>MSTRSARIVVVSSRAAAGVYTDDCGPIIAGWLEQHGFSSVQPQVVADGNPVGEALHDAVNAGVDVIITSGGTGISPTDTTPEHTVAVLDYVIPGLADAIRRSGLPKVPTSVLSRGVCGVAGRTLIINLPGSPGGVRDGLGVLADVLDHALEQIAG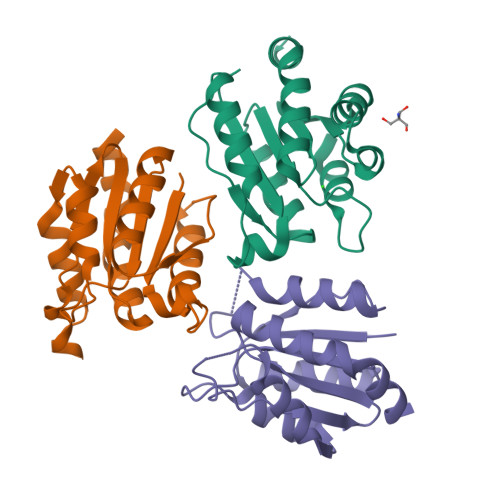GDHPR[3x]> MLAKRIIACLDVKDGRVVKGTNFENLRDSGDPVELGKFYSEIGIDELVFLDITASVEKRKTMLELVEKVAEQIDIPFTVGGGIHDFETASELILRGADKVSINTAAVENPSLITQIAQTFGSQAVVVAIDAKRVDGEF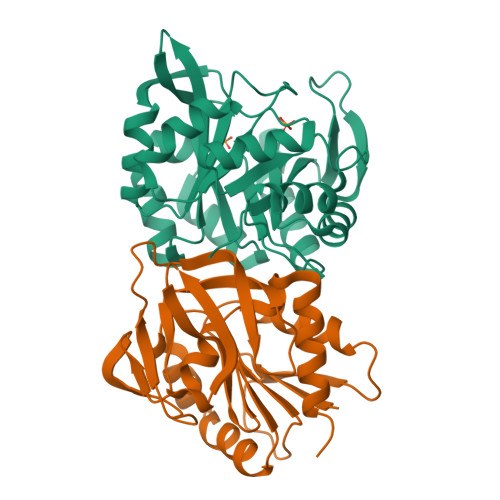MVFTYSGKKNTGILLRDWVVEVEKRGAGEILLTSIDRDGTKSGYDTEMIRFVRPLTTLPIIASGGAGKMEHFLEAFLAGADAALAASVFHFREIDVRELKEYLKKHGVNVRLEGL;> MRIGIISVGPGNIMNLYRGVKRASENFEDVSIELVESPRNDLYDLLFIPGVGHFGEGMRRLRENDLIDFVRKHVEDERYVVGVCLGMQLLFEESEEAPGVKGLSLIEGNVVKLRSRRLPHMGWNEVIFKDTFPNGYYYFVHTYRAVCEEEHVLGTTEYDGEIFPSAVRKGRILGFQFHPEKSSKIGRKLLEKVIECSLSRR>[5x]MGNNLMQTDLSVWGMYQHADIVVKCVMIGLILASVVTWAIFFSKSVEFFNQKRRLKREQQLLAEARSLNQANDIAADFGSKSLSLHLLNEAQNELELSEGSDDNEGIKERTSFRLERRVAAVGRQMGRGNGYLATIGAISPFVGLFGTVWGIMNSFIGIAQTQTTNLAVVAPGIAEALLATAIGLVAAIPAVVIYNVFARQIGGFKAMLG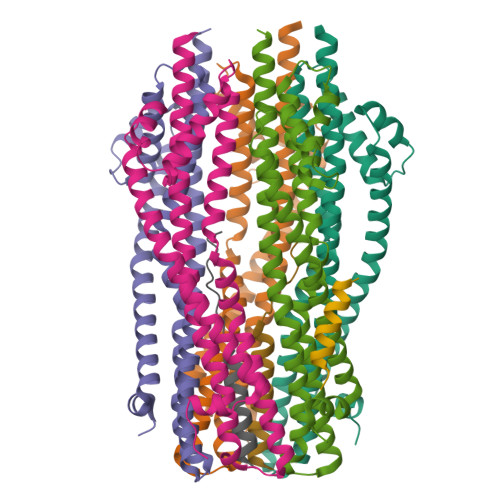DVAAQVLLLQSRDLDLEASAAAHPVRVAQKLRAG;> MTLDLPRRFPWPTLLSVCIHGAVVAGLLYTSVHQVIELPAPAQPISVTMVTPADLEPPQAVQPPPEPVVEPEPEPEPIPEPPKEAPVVIEKPKPKPKPKPKPVKKVQEQPKRDVKPVESRPASPFENTAPARLTSSTATAATSKPVTSVASGPRALSRNQPQYPARAQALRIEGQVKVKFDVTPDGRVDNVQILSAKPANMFEREVKNAMRRWRYEPGKPGSGIVVNILFKINGTTEIQGGGSENLYFQGGSAWSHPQFEK;>MAMHLNENLDDNGEMHDINVTPFIDVMLVLLIIFMVAAPLATVDVKVNLPASTSTPQPRPEKPVYLSVKADNSMFIGNDPVTDETMITALNALTEGKKDTTIFFRADKTVDYETLMKVMDTLHQAGYLKIGLVGEETAKAKENLYFQGNAGSGHHHHHHHHHH[2x]> DSFSLLSQITPHQRCSFYAQVI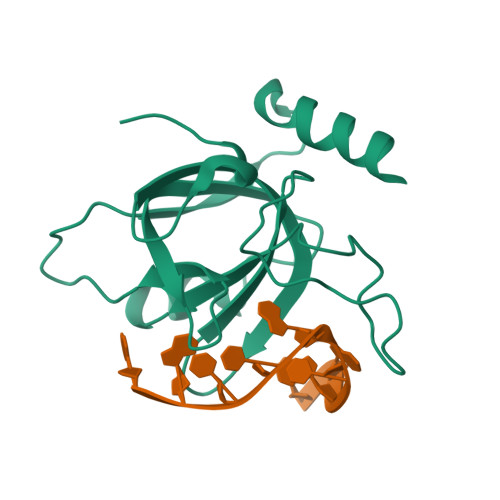KTWYSDKNFTLYVTDYTENELFFPMSPYTSSSRWRGPFGRFSIRCILWDEHDFYCRNYIKEGDYVVMKNVRTKIDHLGYLECILHGDSAKRYNMSIEKVDSEEPELNEIKSRKRLYV> MAEEANKDADISSLSLSLDPEIIGGQNNFLENNLQQIFQKIIQERGPFRDLKEEDLQKELQKESIKDESSAKSSETENVLEFATLDSKRNVNDTEVESMDSQAYKKELIEQIMIAQTECSLALDMTSLLLSKFKENSIETISPFLKSTVPPSSLQFSRSQPPESKESDATLAKCWKEKSLTSSCKFLFEAKERLTSVVETEHEYYTELVKVKEASWPLFNSQGSNHLSVQYSCLGGISLGLGLIRMKPESKSFEVQSSLLYSQAALKISILNKDRDEIGSSTWSWPSQ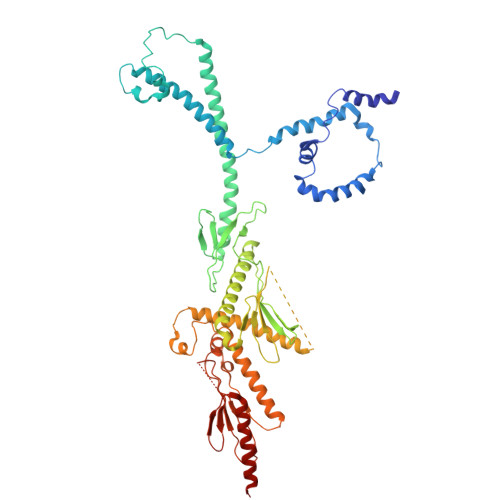NCNSVLLKDIYKLQEILFEMDIWNSLLQEAQSCGNQGVNFTGDEILVPISDDHVVRITLETSSKNTESGFTEDKKSNEDTSTNFVTIKQEKELLKCLCDTLNAIAHILFLKHCRKSDRRSQQPELYMAIDANAPLILRPLIFYYNLNQESLEFQRWLKQRDISFKFMPNYPWEKAKDFLELENSLSINRLSISWRIMVSNFEPAIFIQHTPTLHGTDKSVWRCKDQYSSNQFSSLKNVCQYIEHHINSLSRRSKKTE>[8x]GSTGSMVKSGKARAHTNIALIKYWGKADETYIIPMNNSLSVTLDRFYTETKVTFDPDFTEDCLILNGNEVNAKEKE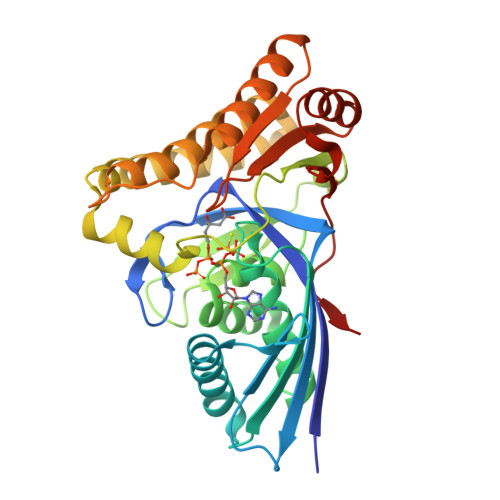KIQNYMNIVRDLAGNRLHARIESENYVPTAAGLASSASAYAALAAACNEALSLNLSDTDLSRLARRGSGSASRSIFGGFAEWEKGHDDLTSYAHGINSNGWEKDLSMIFVVINNQSKKVSSRSGMSLTRDTSRFYQYWLDHVDEDLNEAKEAVKNQDFQRLGEVIEANGLRMHATNLGAQPPFTYLVQESYDAMAIVEQCRKANLPCYFTMAAGPNVKVLVEKKNKQAVMEQFLKVFDESKIIASDIISSGVEIIK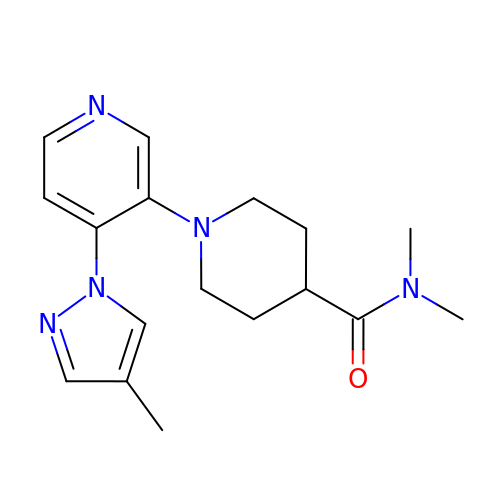N,N-dimethyl-1-[4-(4-methyl-1H-pyrazol-1-yl)pyridin-3-yl]piperidine-4-carboxamide | C17 H23 N5 O | MYSVNUHQXQZBQE-UHFFFAOYSA-N DEC-205 (CD205), a member of the macrophage mannose receptor protein family, is the prototypic endocytic receptor of dendritic cells, whose ligands include phosphorothioated cytosine–guanosine oligonucleotides, a motif often seen in bacterial or viral DNA. The MR protein family is characterized by a conserved domain architecture that comprises an N-terminal cysteine-rich (CysR) domain, a fibronectin type II (FNII) domain, and 8 or 10 contiguous C-type lectin-like domains (CTLDs). Here, DEC-205 is thought to function as a promiscuous endocytic receptor that captures a diverse repertoire of foreign and self-antigens and internalize them for antigen processing and cross-presentation. Namely, DEC-205, PLA2R, and the avian IgY receptor FcRY are all reported to exist in a compact conformation at low pH and transition to an extended state under basic conditions, although the mechanism of such rearrangements are unknown.

Given that DEC-205 adopts a compact conformation at low pH, we prepared samples for single-particle cryo-EM data collection at pH 6.0 consistent with early late endosomes where DEC-205 traffics. The structure of the DEC-205 ECD was determined to a resolution of 3.2 Å. The DEC-205 ECD domains pack tightly together presenting in a lemniscate (∞) with dimensions of roughly 110 × 70 × 70 Å. Each of the tightly packed DEC-205 ECDs could be built from the N-terminal CysR (R30) to CTLD8 (E1383); however, the C-terminal CTLD 9 and 10 were invisible in the reconstruction. The centrally located and globular CysR and FNII domains lead into a compact 60 Å ring with a central cavity of ∼15 Å comprised of a counter-clockwise arrangement of CTLD1 through to CTLD4. The second and slightly larger ∼65 Å ring comprises of a clockwise arrangement of CTLD5 through to CTLD8. Here, the central cavity of the second ring was occupied by an extended loop of CTLD5. Each of the CTLDs adopted a compact β2-3 loop architecture with the exclusion of CTLD5 that stood in stark contrast with a fully extended β2-3 loop that played a role in coordinating the secondary CTLD ring and thus in stabilizing the DEC-205 ECD. Most striking was the extended β2-3 loop of CTLD5, which acted as a “recruitment hub”, whereby it co-ordinated several domains within the secondary ring including CTLDs 6, 7, and 8. Here, R895 seemed to tether the loop apex via sidechain interaction with a neutral pocket composed of L1172, N1173, and Q1193 within CTLD7 with peripheral interaction between W893 and H1183, which further stabilized the extended long-loop conformation.

> RAANDPFTIVHGNTGKCIKPVYGWIVADDCDETEDKLWKWVSQHRLFHLHSQKCLGLDITKSVNELRMFSCDSSAMLWWKCEHHSLYGAARYRLALKDGHGTAISNASDVWKKGGSEESLCDQPYHEIYTRDGNSYGRPCEFPFLIDGTWHHDCILDEDHSGPWCATTLNYEYDRKWGICLKPENGCEDNWEKNEQFGSCYQFNTQTALSWKEAYVSCQNQGADLLSINSAAELTYLKEKEGIAKIFWIGLNQLYSARGWEWSDHKPLNFLNWDPDRPSAPTIGGSSCARMDAESGLWQSFSCEAQLPYVCRKPLNNTVELTDVWTYSDTRCDAGWLPNNGFCYLLVNESNSWDKAHAKCKAFSSDLISIHSLADVEVVVTKLHNEDIKEEVWIGLKNINIPTLFQWSDGTEVTLTYWDENEPNVPYNKTPNCVSYLGELGQWKVQSCEEKLKYVCKRKGEKLNDASSDKMCPPDEGWKRHGETCYKIYEDEVPFGTNCNLTITSRFEQEYLNDLMKKYDKSLRKYFWTGLRDVDSCGEYNWATVGGRRRAVTFSNWNFLEPASPGGCVAMSTGKSVGKWEVKDCRSFKALSICKKMSGPLGPEEASPKPDDPCPEGWQSFPASLSCYKVFHAERIVRKRNWEEAERFCQALGAHLSSFSHVDEIKEFLHFLTDQFSGQHWLWIGLNKRSPDLQGSWQWSDRTPVSTIIMPNEFQQDYDIRDCAAVKVFHRPWRRGWHFYDDREFIYLRPFACDTKLEWVCQIPKGRTPKTPDWYNPDRAGIHGPPLIIEGSEYWFVADLHLNYEEAVLYCASNHSFLATITSFVGLKAIKNKIANISGDGQKWWIRISEWPIDDHFTYSRYPWHRFPVTFGEECLYMSAKTWLIDLGKPTDCSTKLPFICEKYNVSSLEKYSPDSAAKVQCSEQWIPFQNKCFLKIKPVSLTFSQASDTCHSYGGTLPSVLSQIEQDFITSLLPDMEATLWIGLRWTAYEKINKWTDNRELTYSNFHPLLVSGRLRIPENFFEEESRYHCALILNLQKSPFTGTWNFTSCSERHFVSLCQKYSEVKSRQTLQNASETVKYLNNLYKIIPKTLTWHSAKRECLKSNMQLVSITDPYQQAFLSVQALLHNSSLWIGLFSQDDELNFGWSDGKRLHFSRWAETNGQLEDCVVLDTDGFWKTVDCNDNQPGAICYYSGNETEKEVKPVDSVKCPSPVLNTPWIPFQNCCYNFIITKNRHMATTQDEVHTKCQKLNPKSHILSIRDEKENNFVLEQLLYFNYMASWVMLGITYRNKSLMWFDKTPLSYTHWRAGRPTIKNEKFLAGLSTDGFWDIQTFKVIEEAVYFHQHSILACKIEMVDYKEEYNTTLPQFMPYEDGIYSVIQKKVTWYEALNMCSQSGGHLASVHNQNGQLFLEDIVKRDGFPLWVGLSSHDGSESSFEWSDGSTFDYIPWKGQTSPGNCVLLDPKGTWKHEKCNSVKDGAICYKPTKSKKLSRLTYSSRCPAAKENGSRWIQYKGHCYKSDQALHSFSEAKKLCSKHDHSATIVSIKDEDENKFVSRLMRENNNITMRVWLGLSQHSVDQSWSWLDGSEVTFVKWENKSKSGVGRCSMLIASNETWKKVECEHGFGRVVCKVPLGPDYTAIAIIVATLSILVLMGGLIWFLFQRHRLHLAGFSSVRYAQGVNEDEIMLPSFHD2-hydroxy-N'-[(Z)-(2-hydroxynaphthalen-1-yl)methylidene]benzohydrazide 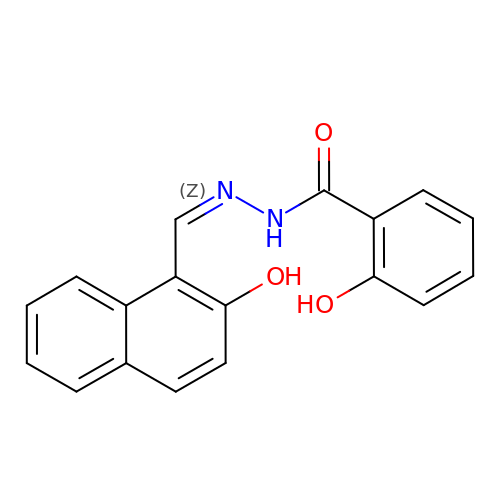| C18 H14 N2 O3 | ZZSJOLDICPVVAV-ODLFYWEKSA-N> LVEQEQTLENYIHAGAYRDAIVLALQLNHPGRLLNLFTNVVTTRNPDPDSLTGLKAVDDVLAKLSDEQIFQLLLRLRDWNTNARTAPVAQR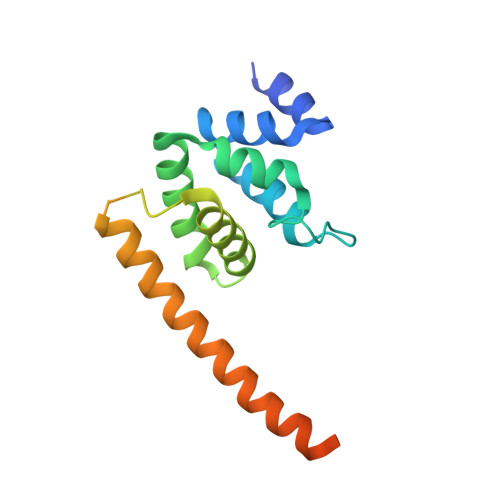VLWALFKSHPANKLSSLSVKGARGHKSLNEVLDAIKVYTERHYKRIEELVDESYLVEYTLREMDALTPQTEALEAGEDAVIAEA>MFKKLLDNKNLVINPPVFITSILLIVALILTCVLFPEKVGVWFPAAQLAVTSNFGWFFVVTVNVILIFAIYLAFSKFGRIRLGGDDAEPEFTKASWFAMLFSTGMGIGIMFFSIAEPVSHFFNTPRPVDTDIEAAVQAMQFTSLHWGLHAWGIYAMVGLALAFFGFNRKLPMTFRSLFYPFWGERIHGWWGHIIDILSALATVFGLSTSLGLGVIQITAGLEYLYGWEISPMMQAGIILFVIGIATISVFSGLDKGVKILSNANMYIAASFMLLIFILGPTLFIMKGYVENTGAYLANFIDISTWNDTYLGSGWQNVWTIFYWAWWIAWSPFVGSFIARISKGRTVKEFVLGVLIVPGLITLLWMNVFGGSALHTILSGDVTMIAAVKADVSTALFVFLENFPFTKFLSIVAIILIFSFFITSSDSGSLVVDNITSGS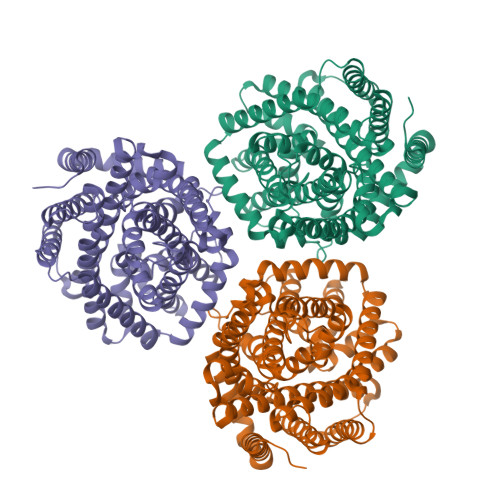NGESPVWQRVFWSFAQGIIAIVLLWGGGLDALQTAVIITGLPFAVILLVMCYSLQKGLKEELAKSSKKAKSKEEKSYKEIIAELLDEPQSKHHHHHHHHHH[3x]> MESLLEKRRQLSRDIGRLKETYEALLARFPNLRFAYKDPEKNWNRNC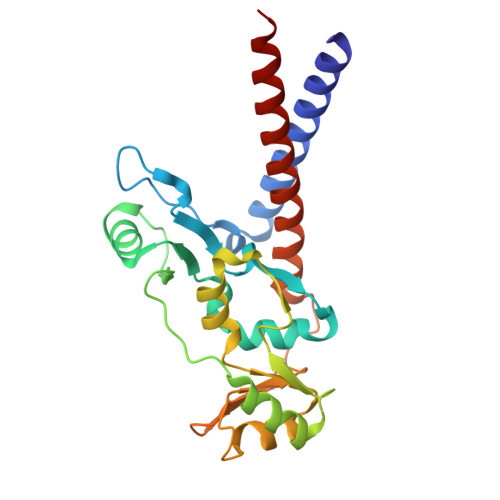VKGLVASLISVKDTSATTALELVAGERLYNVVVDTEVTGKKLLERGELKRRYTIIPLNKISARCIAPETLRVAQNLVGPDNVHVALSLVEYKPELQKAMEFVFGTTFVCDNMDNAKKVAFDKRIMTRTVTLGGDVFDPHGTLSGGARSQAASILTKFQELKDVQDELRIKENELRALEEELAGLKN> MGEEFEKLMKKFENVNKDGEIVEDEDEWEEFFKQEEYVKIPKDRIAVLIGKKGQTKKEIEKRTKTKITIDSETGEVWITSTKETEDPLAVWKARDIVLAIGRGFSPERAFRLLNEGEYLEIINLTDIIIGNEKNALPRVRGRIIGRKGRTRQIIEEMSGASVSVYGKTVAIIGNPIQIEIAKTAIEKL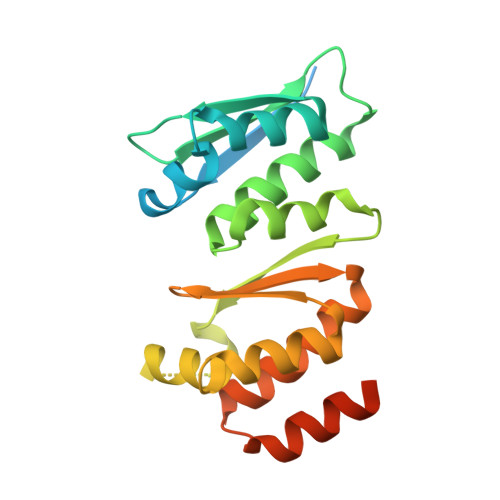ARGSPHGSVYRYLERRKKDLELEGAMYYENL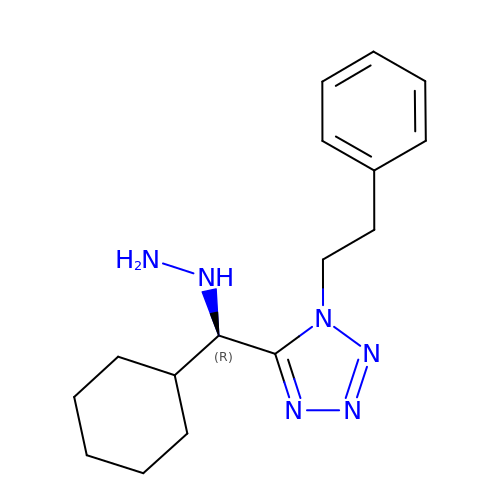[(~{R})-cyclohexyl-[1-(2-phenylethyl)-1,2,3,4-tetrazol-5-yl]methyl]diazane | C16 H24 N6 | RYAQXBFFYZPWMF-OAHLLOKOSA-N(3R,4S,5R)-3,4,5-TRIHYDROXYCYCLOHEX-1-ENE-1-CARBOXYLIC 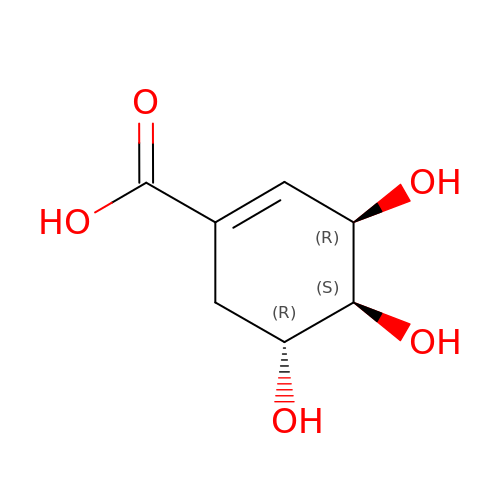ACID | C7 H10 O5 | JXOHGGNKMLTUBP-HSUXUTPPSA-N>[2x]GHAKKPLMEKNKVTQQFSILPGNKAFKGKFTVPGDKSVSHRSIMFGAIAEGTTHVTGFLEGEDALATLQAFRDMGVSIEGPKNGEVTIHGVGMHGLKAPASALYMGNSGTSMRLLSGMLSAQKFDSVMTGDASLSKRPMERIAKPLRLMGAQIQTTGEKGTPPVSITGGQQLKGIQYDLPMASAQVKSGILLAGLWAEGETSV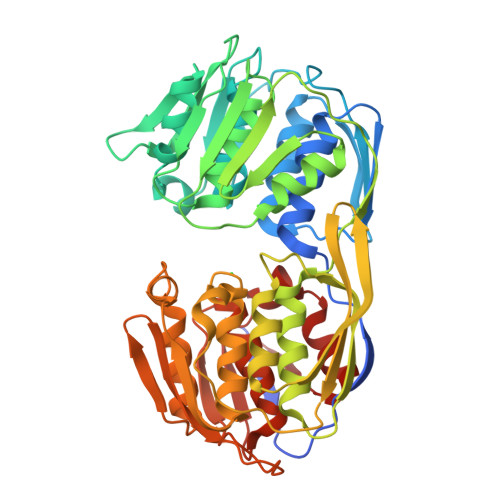TEPEPTRDHTERMLRAFGYDVKTEGNKISLVGGGKLVGTNIQVPSDISSAAFFMVGAAITEGADVVLEAVGINPTRTGVIEILKQMGADLTVENERIAGGEPIADIHIKGSRTLKGIHMPEDQVPLAIDEFPALFIAAACAEGQTVLTGAAELRVKESDRIQVMADGLKIMGIDCTPTEDGIIIEGKGKSGDWSPIFAGGEIESHHDHRIAMSFSMAGLRTSGPITIHGTETVATSFPTFTELANRAGLTIEVSQ> MERKQKNSLFNYIYSLMDVRGKFLFFSMLFITSLSSIIISISPLILAKITDLLSGSLSNFSYEYLVLLACLYMFC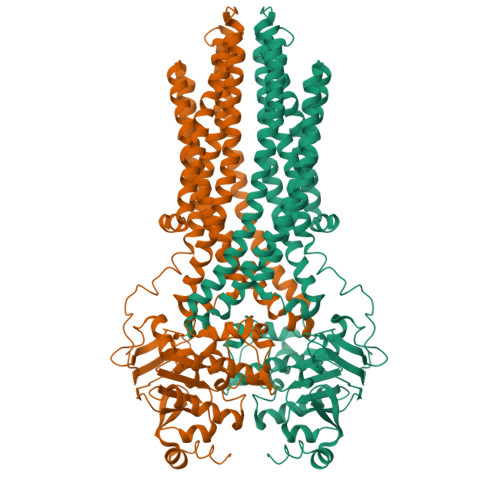VISNKASVFLFMILQSSLRINMQKKMSLKYLRELYNENITNLSKNNAGYTTQSLNQASNDIYILVRNVSQNILSPVIQLISTIVVVLSTKDWFSAGVFFLYILVFVIFNTRLTGSLASLRKHSMDITLNSYSLLSDTVDNMIAAKKNNALRLISERYEDALTQENNAQKKYWLLSSKVLLLNSLLAVILFGSVFIYNILGVLNGVVSIGHFIMITSYIILLSTPVENIGALLSEIRQSMSSLAGFIQRHAENKATSPSIPFLNMERKLNLSIRELSFSYSDDKKILNSVSLDLFTGKMYSLTGPSGSGKSTLVKIISGYYKNYFGDIYLNDISLRNISDEDLNDAIYYLTQDDYIFMDTLRFNLRLANYDASENEIFKVLKLANLSVVNNEPVSLDTHLINRGNNYSGGQKQRISLARLFLRKPAIIIIDEATSALDYINESEILSSIRTHFPDALIINISHRINLLECSDCVYVLNEGNIVASGHFRDLMVSNEYISGLASVTE>MSNWPYPRIVAHRGGGKLAPENTLAAIDVGAKYGHKMIEFDAKLSKDGEIFLLHDDNLERTSNGWGVAGELNWQDLLRVDAGSWYSKAFKGEPLPLLSQVAERCREHGMMANIEIKPTTGTGPLTGKMVALAARQLWAGMTPPLLSSFEIDALEAAQQAAPELPRGLLLDEWRDDWRELTA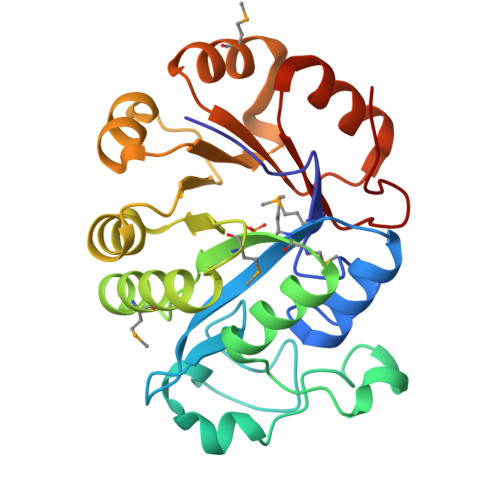RLGCVSIHLNHKLLDKARVMQLKDAGLRILVYTVNKPQHAAELLRWGVDCICTDAIDVIGPNFTAQ[4x]>MAELILNQRPYPRDLGKIVCVGRNYAAHAKELNNPIPSSPILFIKPASSAVPFGPVFSIPKDQGSVHHELEIAILIGKALSRASTEQVAESIAGIGLGLDLTLRDVQDQLKEKGHPWERAKSFDGACPLTEFVAVNLASEDEWQAIGLTLEKNGQFQQQGSSAEMLFPILPLIAHMSEHFSLQPGDVILTGTPAG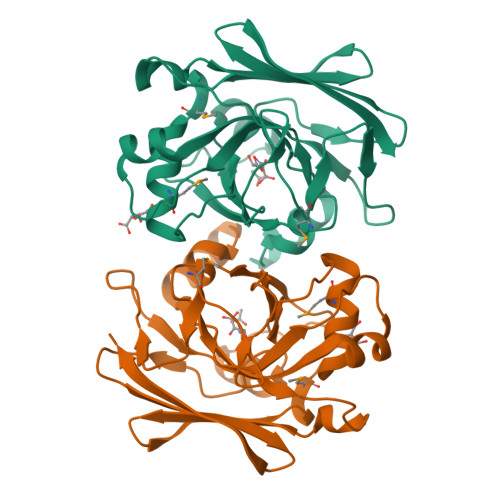VGPLEVGDSLSAKLSLEDNVLLTCDGVVI[6x]> MAHSSATAGPQADYSGEIAELYDLVHQGKGKDYHREAADLAALVRRHSPKAASLLDVACGTGMHLRHLADSFGTVEGLELSADMLAIARRRNPDAVLHHGDMRDFSLGRRFS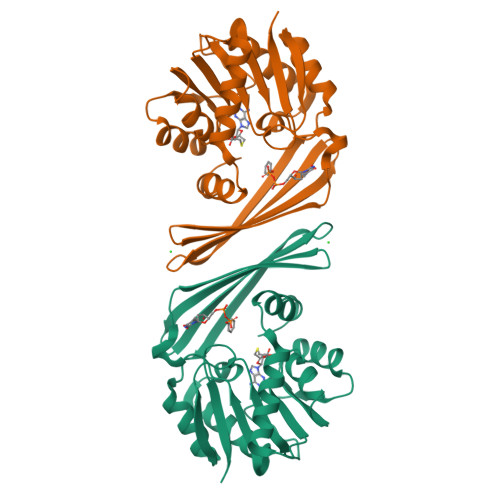AVTCMFSAIGHLAGQAELDAALERFAAHVLPDGVVVVEPWWFPENFTPGYVAAGTVEAGGTTVTRVSHSSREGEATRIEVHYLVAGPDRGITHHEESHRITLFTREQYERAFTAAGLSVEFMPGGPSGRGLFTGLPGAKGETRLEHHHHHH>GAMGSSPSLEQDDGDEETSVVIVGKISFCPKDVLGHGAEGTIVYRGMFDNRDVAVKRILPECFSFADREVQLLRESDEHPNVIRYFCTEKDRQFQYIAIELCAATLQEYVEQKDFAHLGLEPITLLQQTTSGLAHLHSLNIVHRDLKPHNILISMPNAHGKIKAMISDFGLCKKLAVGRHSFSRRSGVPGTEGWIAPEMLSEDCKENPTYTVDIFSAGCVFYYVISEGSHPFGKSLQRQANILLGACSLDCLHPEKHEDVIARELIEKMIAMDPQKRPSAKHVLKHPFFWSLEKQLQFFQDVSDRIEKESLDGPIVKQLERGGRAVVKMDWRENITVPLQTDLRKFRTYKGGSVRDLLRAMRNKKHHYRELPAEVRETLGSLPDDFVCYFTSRFPHLLAHTYRAMELCSHERLFQPYYFHE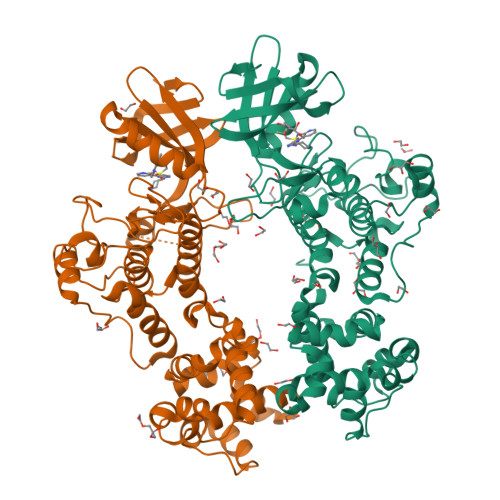PPEPQPPVTPDAL[2x]> GGIKMDTQFYDSFTFDNVKYSLYDNVYLFKSGESEPYIG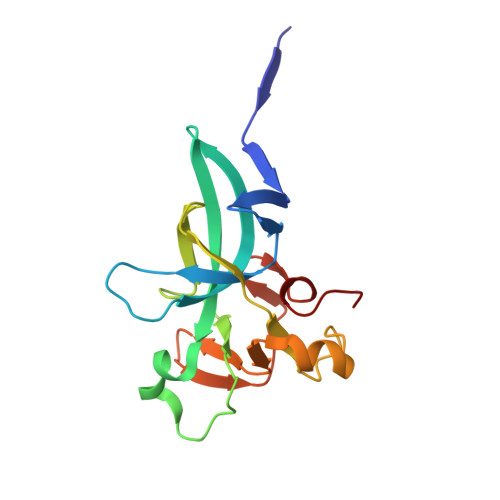KIIKIWQQNQAKKVKILWFFLPDEIRKHLSGPVMEKEIFLACGEGVGLADINPLEAIGGKCTVLCISKDERNRQPSPRELAMADYIFYRFFDVNSCTLSEQLPEKIAGVEGNLLLNSKVE> GSGSMISIFIAEDQQMLLGALGSLLNLED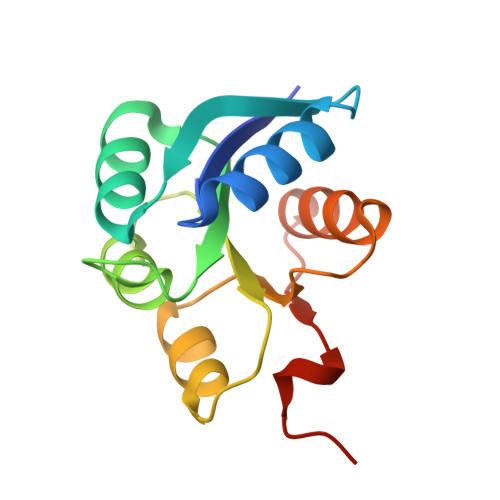DMEVVGKGTTGQDAVDFVKKRQPDVCIMDIEMPGKTGLEAAEELKDTGCKIIILTTFARPGYFQRAIKAGVKGYLLKDSPSEELANAIRSVMNGKRIYAPELMEDLYSEA>[6x]MAHHHHHHMATPHNSAKVGDFAETVLMCGDPLRAKLIADNYLENAKQVNSVRGMLGFTGTYKGKPLSVMGH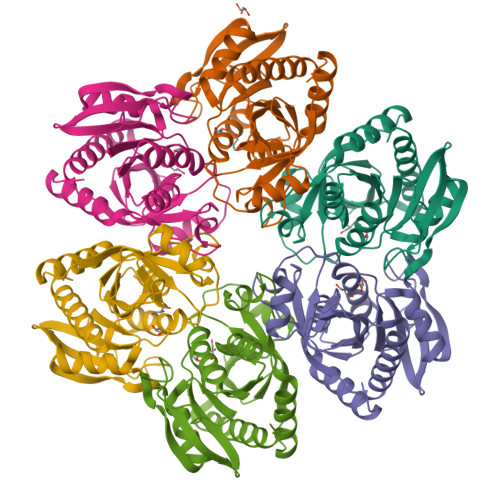GMGIPSISIYAEELYNVYKVKTIIRVGTCGTVDPNVHVRDVCIVTASGTDSNVNRMRLLGHDFPATANFEVVSALVESAKALNIPTQVGKAYSTDIFYSKEQGLNEALAQYHFIAVEMESAGLFPIADYYGARAGCICTVSDHIITHESATPEERQTSFQNMIKIALEATLKL>MMLSLNNLQNIIYNPVIPFVGTIPDQLDPGTLIVIRGHVPSDADRFQVDLQNGSSMKPRADVAFHFNPRFKRAGCIVCNTLINEKWGREEITYDTPFKREKSFEIVIMVLKDKFQVAVNGKHTLLYGHRIGPEKIDTLGIYGKVNIHSIGFSFSSHMRLPFAARLNTPMGPGRTVVVKGEVNANAKSFNVDLLAGKSKDIALHLNPRLNIKAFVRNSFLQESWGEEERNITSFPFSPGMYFEMII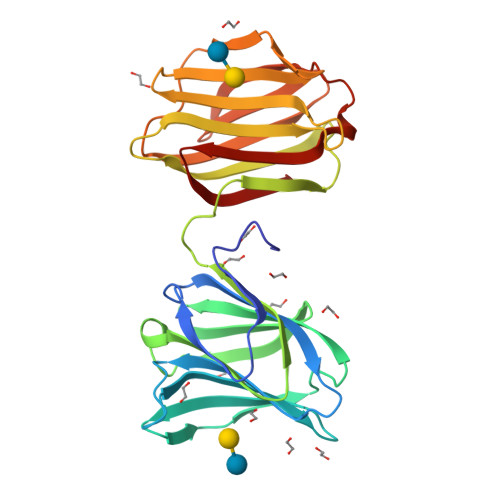YCDVREFKVAVNGVHSLEYKHRFKELSSIDTLEINGDIHLLEVRSW[2x]>[4x]MAKKTSSKGKLPPGPSPLPVLGNLLQMDRKGLLRSFLRLREKYGDVFTVYLGSRPVVVLCGTDAIREALVDQAEAFSGRGKIAVVDPIFQGYGVIFANGERWRALRRFSLATMRDFGMGKRSVEERIQEEARCLVEELRKSKGALLDNTLLFHSITSNIICSIVFGKRFDYKDPVFLRLLDLFFQSFSLISSFSSQVFELFSGFLKYFPGTHRQIYRNLQEINTFIGQSVEKHRATLDPSNPR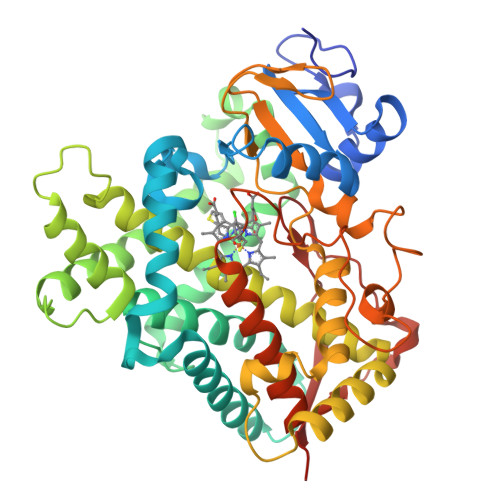DFIDVYLLRMEKDKSDPSSEFHHQNLILTVLSLFFAGTETTSTTLRYGFLLMLKYPHVTERVQKEIEQVIGSHRPPALDDRAKMPYTDAVIHEIQRLGDLIPFGVPHTVTKDTQFRGYVIPKNTEVFPVLSSALHDPRYFETPNTFNPGHFLDANGALKRNEGFMPFSLGKRICLGEGIARTELFLFFTTILQNFSIASPVPPEDIDLTPRESGVGNVPPSYQIRFLARHHHH1-(4-bromo-2-chlorophenyl)-3-methylthiourea | C8 H8 Br Cl 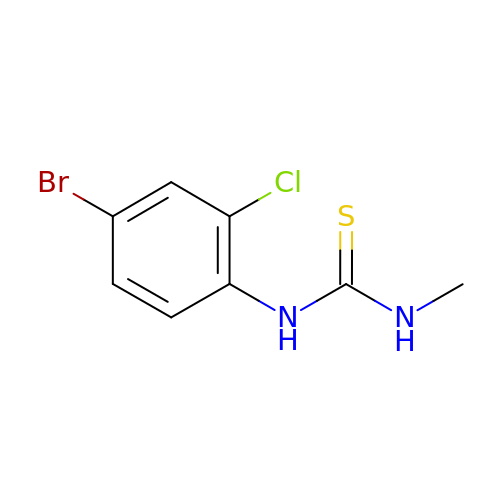N2 S | LXSVLJOSFCRPPA-UHFFFAOYSA-N> GSHMEKEADEARRQIVSNALISEIAGIVDFVAEEQITVIEQGIEKEITNPLYEQSSGIPYINRTTNKDLNSTMSTNASEFINWGAGTSTRIFFTRKYCISTGTQGNYEFSKDYIPCEEPAILSNSDLKIDRIDFVATDNTV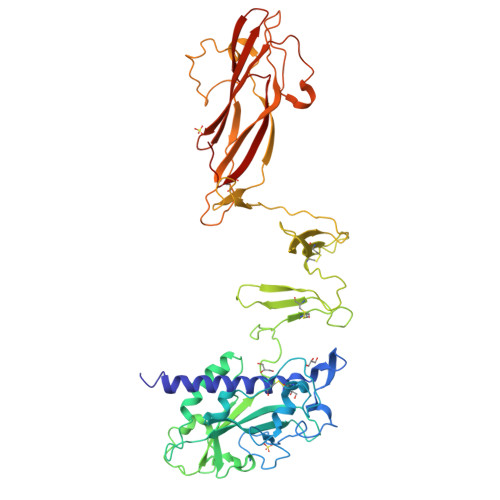GSAIERVDFILTFDKSNANESFYFSNYVSSLEKAAEQHSISFKDIYVVERNSSGAAGWRLTTISGKPLTFSGLSKNIGSLDKTKNYGLRLSIDPNLGKFLRADGRVGADKLCWNIDNKMSGPCLAADDSGNNLVLTKGKGAKSNEPGLCWDLNTGTSKLCLTQIEGKDNNDKDASLIKLKDDNGNPATMLANILVEEKSMTDSTKKELRTIPNTIYAAFSNSNASDLVITNPGNYIGNVTSEKGRIELNVQDCPVSPDGNKLHPRLSASIASIVADTKDSNGKYQADFSSLAGNRNSGGQLGYLSGTAIQVNQSGSKWYITATMGVFDPLTNTTYVYLNPKFLSVNITTWCSTEPQT> MTDKLIRELLIDVKQKGATRTAKSIENVSDALENAAAASELTNEQLGKMPRTLYSIERAADRAAKSLTKMQASRGMAGITKSIDGIGDKLDYLAIQLIEVTDKLEIGFDGVSRSVKAMGNDVAAATEKVQDRLYDTNRALGGTSKGFNDTAGAAGRASRALGNTSGSARGATRDFAAMAKIGGRLPIMYAALASNVFVLQTAFESLKVGDQLNRLEQFGTIVGTMTGTPVQTLALSLQNATNGAISFEEAMRQASSASAYGFDSEQLEQFGLVARRAAAVLGVDMTDALNRVIKGVSKQEIELLDELGVTIRLNDAYENYVKQLNATSTGIKYTVDSLTTYQKQQAYANEVIAESTRRFGYLDDALKATSWEQFAANANSALRSLQQSAATYLNPVMDTLNTFLYQTKSSQMRVSAMARSASAKTTPAENVTALIENAVGAREDLDTYLKESEERVKKAQELKQQLDDLKAKQAATAPIANALTAGGIGGDESNKLVVQLTNELARQNKEIEERTKTEKVLRQAVQDTGEALLRNGKLAEQLGAKMKYADTAVPGDKGVFEVDPNNLKAVSEIQKNFDFLKKSSSDTANNIRMAASSITNAKKASSDLNSVVKAVEDTSKVTGQSADTLVKNLNLGFSSLDQMKAAQKGLSEYVTAMDKSEQNALEVAKRKDEVYNQTKDKAKAEAAAREVLL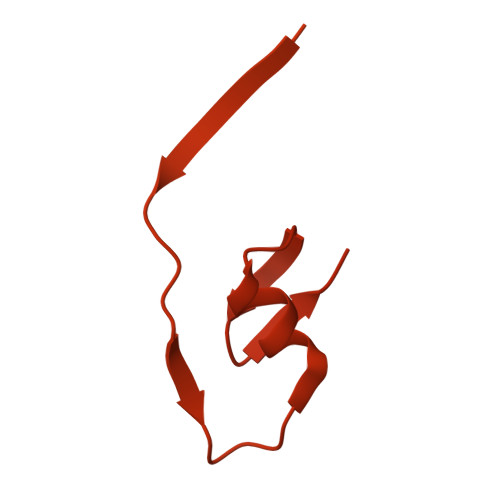RQQQEQLTAAKALLAINPNDPEALKQVAKIETEILNTKAQGFENAKKTKDYTDKILGVDREIALLNDRTMTSTQYRLAQLRLELQLEQEKTELYSKQADGQAKVEQSRRAQAQISREIWEAEKQGTASHVSALMDALEVSQTQRNVTGQSQILTERLSILQQQLELSKGNTEEELKYRNEIYKTSAALEQLKKQRESQMQQQVGSSVGATYTSTTGLIGEDKDFADMQNRMASYDQAISKLSELNSEATAVAQSMGNLTNAMIQFSQGSLDTTSMIASGMQTVASMIQYSTSQQVSAIDQAIAAEQKRDGKSEASKAKLKKLEAEKLKIQQDAAKKQIIIQTAVAVMQAATAVPYPFSIPLMVAAGLAGALALAQASSASGMSSIADSGADTTQYLTLGERQKNVDVSMQASSGELSYLRGDKGIGNANSFVPRAEGGMMYPGVSYQMGEHGTEVVTPMVPMKATPNDQLSDGSKTTSGRPIILNISTMDAASFRDFASNNSTAFRDAVELALNENGTTLKSLGNS> MSNYPLHQACMENEFFKVQELLHSKPSLLLQKDQDGRIP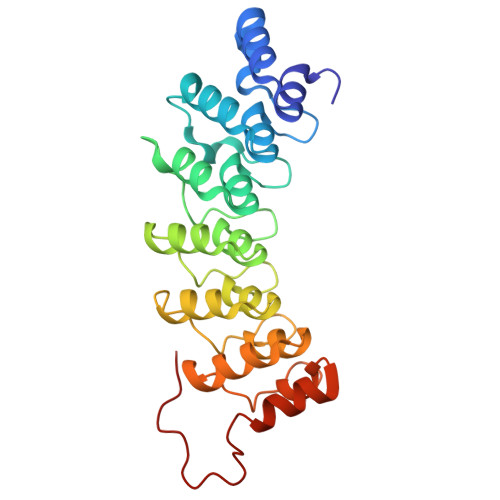LHWSVSFQAHEITSFLLSKMENVNLDDYPDDSGWTPFHIACSVGNLEVVKSLYDRPLKPDLNKITNQGVTCLHLAVGKKWFEVSQFLIENGASVRIKDKFNQIPLHRAASVGSLKLIELLCGLGKSAVNWQDKQGWTPLFHALAEGHGDAAVLLVEKYGAEYDLVDNKGAKAEDVALNEQVKKFFLNNVVDKLAAALEHHHHHH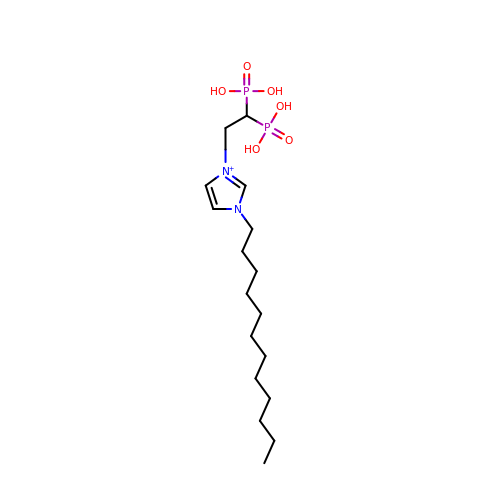3-(2,2-diphosphonoethyl)-1-dodecyl-1H-imidazol-3-ium | C17 H35 N2 O6 P2 | LPGGFVFFIYFOME-UHFFFAOYSA-O>MKPHPWFFGKIPRAKAEEMLSKQRHDGAFLIRESESAPGDFSLSVKFGNDVQHFKVLRDGAGKYFLWVVKFNSLNELV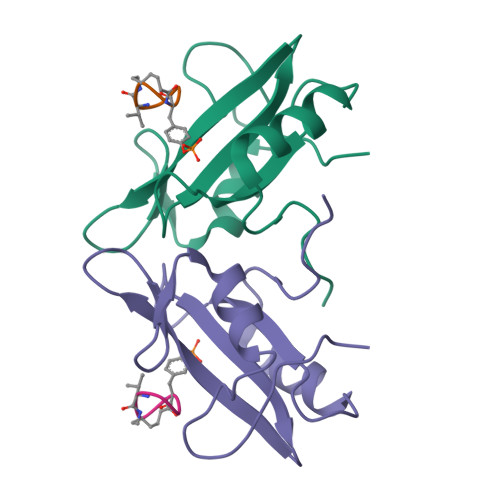DYHRSTSVSRNQQIFLRDIE[3x];>[3x]YVNVX> MASSDLEQLC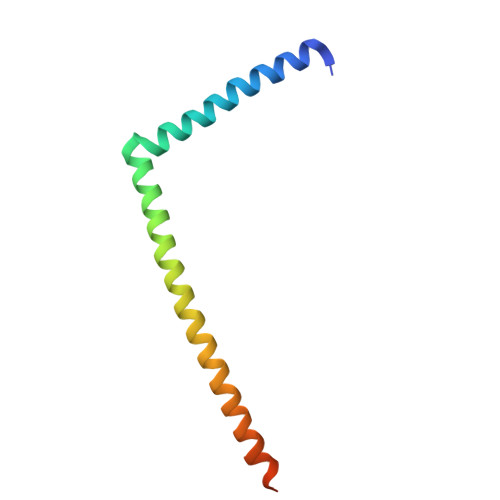SHVNEKIGNIKKTLSLRNCGQEPTLKTVLNKIGDEIIVINELLNKLELEIQYQEQTNNSLKELCESLEEDYKDIEHLKENV> MIKVKSPGRVNLIGEHTDYTYGYVMPMAI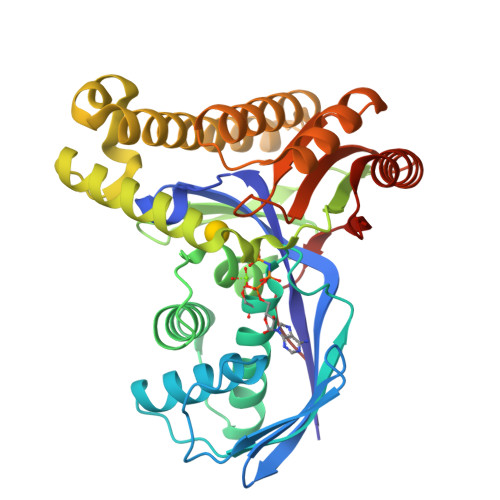NLYTKIEAEKHGEVILYSEHFGEERKFSLNDLRKENSWIDYVKGIFWVLKESDYEVGGIKGRVSGNLPLGAGLSSSASFEVGILETLDKLYNLKLDSLSKVLLAKKAENEFVGVPCGILDQFAVVFGREGNVIFLDTHTLDYEYIPFPKDVSILVFYTGVRRELASSEYAERKHIAEESLKILGKGSSKEVREGELSKLPPLHRKFFGYIVRENARVLEVRDALKEGNVEEVGKILTTAHWDLAKNYEVSCKELDFFVERALKLGAYGARLTGAGFGGSAIALVDKEDAETIGEEILREYLKRFPWKARHFIVEPSDGVGI>MHHHHHAIYNVEVETGDREHAGTDATITIRITGAKGRTDYLKLDKGSFEAGSKEQYTVQGFDVGDIQLIELHSDGGGYWSGDPDWFVNRVIIISSTQDRVYSFPCFRWVIKDMVLFPGEATLPFNEVPAIVSEQRQKELEQRKLTYQWDYVSDDMPGNIKAKTHDDLPRDVQFTDEKSRSYQESRKAALVNLGIGSLFTMFENWDSYDDYHILYRNWILGGTPNMADRWHEDRWFGYQFLNGANPVILTRCDALPSNFPVTNEHVNASLDRGKNLDEEIKDGHIYIVDFKVLVGAKSYGGPVLEDIGYKVPDHLKHDEADIRYCAAPLALFYVNKLGHLMPIAIQINQEPGPENPIWTPHEENEHDWMMAKFWLGVAESNFHQLNTHLLRTHLTTESFALSTWRNLASAHPIFKLLQPHIYGVLAIDTIGRKELWGSGGIVDQSLSLGGGGHVTFMEKCFKEVNLQDYHLPNALKKRGVDDPSKLPGFYYRDDGLALWEAIETFIGEIIAIFYKNDDDVKRDNEIQSWIYDVHKNG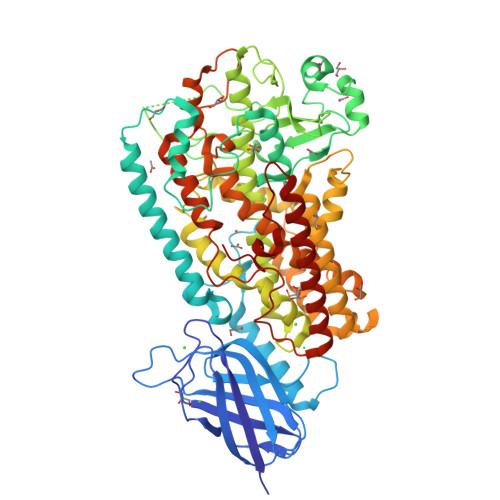WRVNPGHQDHGVPASFESREQLKEVLTSLVFTFSCQHAAVNFSQKDHYGFTPNAPAILRHPPPKKKGEATLQSILSTLPSKSQAAKAIATVYILTKFSEDERYLGNYSATAWEDKDALDAINRFQDKLEDISKKIKQRNENLEVPYIYLLPERIPNGTAI[4x]> GSHGMRSVSGQVVCVTGAGGFIASWLVKILLEKGYTVRGTVRNPDDPKNGHLRELEGAKERLTLCKADLLDYQSLREAINGCDGVFHTASPVTDDPEQMVEPAVIGTKNVINAAAEANVRRVVFTSSIGAVYMDPNRDPETVVDETCWSDPDFCKNTKNWYCYGKMVAEQAAWEEAKEKGVDLVVINPVLVQGPL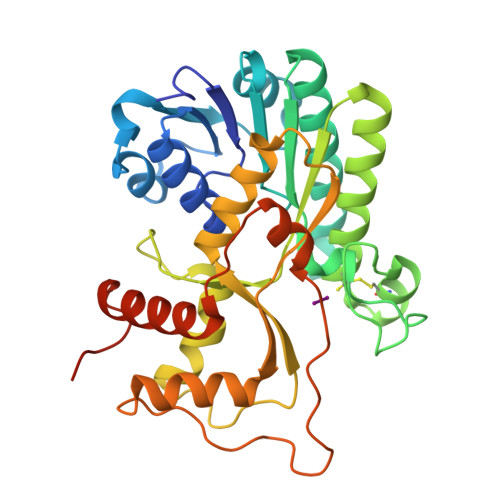LQTTVNASVLHILKYLTGSAKTYANSVQAYVDVKDVALAHILLYETPEASGRYLCAESVLHRGDVVEILSKFFPEYPIPTKCSDVTKPRVKPYKFSNQKLKDLGLEFTPVKQCLYETVKSLQEKGHLPIPTQKDEPIIRIQP> MGCDRNCGLIAGAVIGAVLAVFGGILMPVGDLLIQKTIKKQVVLEEGTIAFKNWVKTGTEVYRQFWIFDVQNPQEVMMNSSNIQVKQRGPYTYRVRFLAKENVTQDAEDNTVSFLQPNGAIFEPSLSVGTEADNFTVLNLAVAAASHIYQNQFVQMILNSLINKSKSSMFQVRTLRELLWGYRDPFLSLVPYPVTTTVGLFYPYNNTADGVYKVFNGKDNISKVAIIDTYKGKRNLSYWESHCDMINGTDAASFPPFVEKSQVLQFFSSDICRSIYAVFESDVNLKGIPVYRFVLPSKAFASPVENPDNYCFCTEKIISKNCTSYGVLDISKCKEGRPVYISLPHFLYASPDVSEPIDGLNPNEEEHRTYLDIEPITGFTLQFAKRLQVNLLVKPSEKIQVLKNLKRNYIVPILWLNETGTIGDEKANMFRSQVTGKINLLGLIEMILLSVGVVMFVAFMISYCACRSKTIK;> EDKIMSYNAFFWMWVHDMLIDSIKWRDEHGRCINKDKGKTCIKGCNKKCISFQKWVEQKKTEWGKIKDHFRKQKDIPKDWTHDDFLQTLLMKDLLLEIIQDTYGDANEIKRIEALLEQAGVGGIDFAALAGLYTKGFVAEKDTTIDKLLQHEQKEADKCLKTHTDDTCPPQEDRSVARS

Unlike other human-infective Plasmodium species, this parasite contains a set of adhesive proteins, the PfEMP1, which are expressed on the surfaces of infected red blood cells, causing them to bind to blood vessels and tissues. To mediate endothelial binding, PfEMP1 proteins contain large extracellular ectodomains consisting of 2–10 copies of two domain types, the Duffy-binding like (DBL) and cysteine-rich interdomain region (CIDR) domains. The scavenger receptor, CD36 binds to many classes of CIDRα domain (CIDRα2-6)2223 and is the host receptor most commonly found to interact with parasite isolates from patients and with laboratory-adapted parasite strains27. CD36 is a cell surface scavenger receptor that plays a role in fatty acid uptake, angiogenesis and phagocytosis.

We coexpressed the ectodomain of CD36 (residues 35–439) together with the MCvar1 CIDRα2.8 domain (residues 576–745 with a C626S mutation to remove an unpaired cysteine). The CD36:CIDRα2.8 complex was subjected to crystallization trials with in situ deglycosylation and proteolysis, allowing a complete data set to be collected to 2.07 Å resolution. The CD36 ectodomain adopts an architecture similar to LIMP-2, with an elongated structure, and is decorated with nine N-linked glycans distributed across the protein surface. While LIMP-2 undergoes a pH-dependent conformational change, with an ‘open' conformation at pH 5.5 and a ‘closed' conformation at pH 7.5, CD36, which was crystallized at pH 8.0, adopts an open conformation. Unlike in LIMP-2, the cavity of CD36 contains two electron density features that resemble the extended hydrocarbon chain of a fatty acid. We therefore modelled palmitic acid into these electron densities and observed a close fit. The PfEMP1 CIDRα2.8 domain therefore binds to the α-helical bundle at the membrane-distal tip of CD36, close to the major entrance (entrance 1) to the hydrophobic cavity and in the region identified previously. The majority of the interaction is mediated by F153 from CD36, which fits into a hydrophobic pocket on the CIDRα2.8 domain surface. Secondary interactions are made by a smaller α-helix (residues 668–678) from the CIDRα2.8 domain (mediating hydrogen bonding to CD36 through E672) and a loop (residues 647–656; again hydrogen bonding, this time through D650). In the structure presented here, the MCvar1 CDRα2.8 domain (crystallized at pH 8.0) adopts the typical compact configuration found in other CIDR domains crystallized around physiological pH, and aligns to the CIDRα1 and γ domains with rmsd of 3.4 and 4.3 Å respectively.> MGSSHHHHHHENLYFQGMMFKKKMLAATLSVGLIAPLASPIQESRANTNIENIGDGAEVIKRTEDVSSKKWGVTQNVQFDFVKDKKYNKDALIVKMQGFINSRTSFSDVKGSGYELTKRMIWPFQYNIGLTTKDPNVSLINYLPKNKIETTDVGQTLGYNIG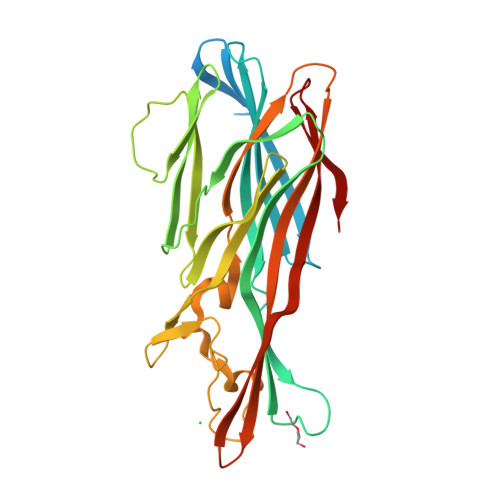GNFQSAPSIGGNGSFNYSKTISYTQKSYVSEVDKQNSKSVKWGVKANEFVTPDGKKSAHDRYLFVQSPNGPTGSAREYFAPDNQLPPLVQSGFNPSFITTLSHEKGSSDTSEFEISYGRNLDITYATLFPRTGIYAERKHNAFVNRNFVVRYEVNWKTHEIKVKGHN> MKWPLLLFTVLLIIGFTLIARAGTISLLSTPPVNPP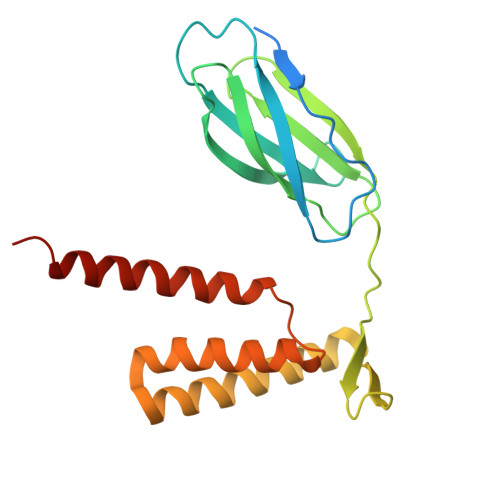AYSYFYIEFQFLPTNNTPQPYAIFVGPNPNNLTEVAEGYTLSNGTGYARVPVINAQTEYVDIVWVNQNYTMFEIFPQIQNATTTVTLSANNNQGFSFSLPTWVSWVIGAVLMLIFMGVGWKFMGPAGLAIFGIFGLFIAMFFGLLPSYLMYVILFIVAIVGARILTKQLGGGEE2-[[2-[[4-[[[3,4-bis(oxidanylidene)-2-[2-(propanoylamino)ethylamino]cyclobuten-1-yl]amino]methyl]phenyl]amino]-5-chloranyl-pyrimidin-4-yl]amino]-~{N}-methyl-benzamide 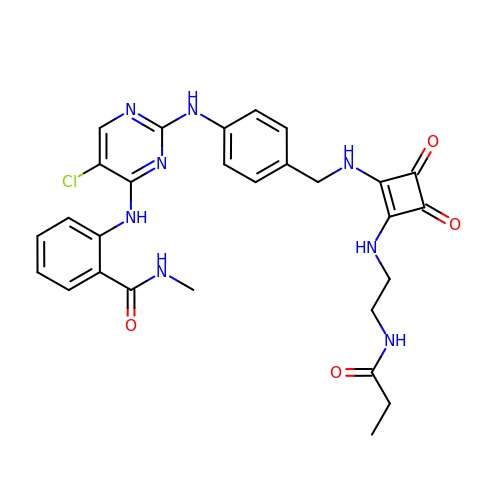| C28 H29 Cl N8 O4 | DZXHGBLWWMPIRK-UHFFFAOYSA-N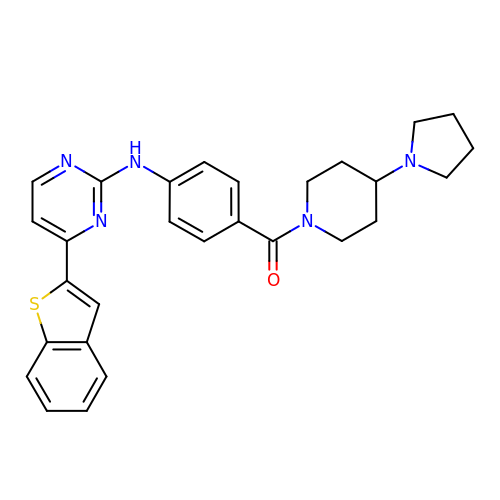(4-{[4-(1-benzothiophen-2-yl)pyrimidin-2-yl]amino}phenyl)[4-(pyrrolidin-1-yl)piperidin-1-yl]methanone | C28 H29 N5 O S | BWZJBXAPRCVCKQ-UHFFFAOYSA-N>[2x]GMAGGRGAPGRGRDEPPESYPQRQDHELQALEAIYGADFQDLRPDACGPVKEPPEINLVLYPQGLTGEEVYV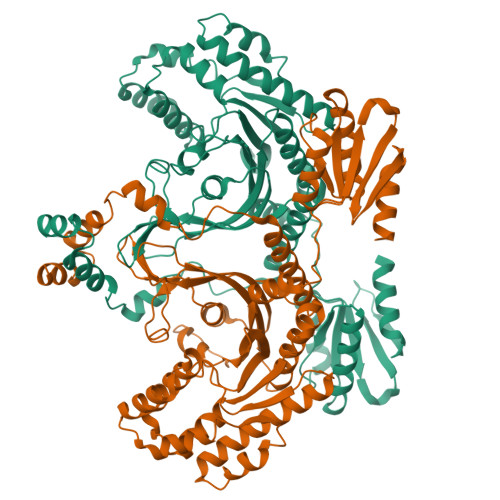KVDLRVKCPPTYPDVVPEIELKNAKGLSNESVNLLKSRLEELAKKHCGEVMIFELAYHVQSFLSEHNKPPPKSFHEEMLERRAQEEQQRLLEAKRKEEQEQREILHEIQRRKEEIKEEKKRKEMAKQERLEIASLSNQDHTSKKDPGGHRTAAILHGGSPDFVGNGKHRANSSGRSRRERQYSVCNSEDSPGSCEILYFNMGSPDQLMVHKGKCIGSDEQLGKLVYNALETATGGFVLLYEWVLQWQKKMGPFLTSQEKEKIDKCKKQIQGTETEFNSLVKLSHPNVVRYLAMNLKEQDDSIVVDILVEHISGVSLAAHLSHSGPIPVHQLRRYTAQLLSGLDYLHSNSVVHKVLSASNVLVDAEGTVKITDYSISKRLADICKEDVFEQTRVRFSDNALPYKTGKKGDVWRLGLLLLSLSQGQECGEYPVTIPSDLPADFQDFLKKCVCLDDKERWSPQQLLKHSFINPQPKMPLVEQSPEDSEGQDYVETVIPSNRLPSAAFFSETQRQFSRYFIEFEELQLLGKGAFGAVIKVQNKLDGCCYAVKRIPINPASRQFRRIKGEVTLLSRLHHENIVRYYNAWIERHERPAGPGTPPPDSGPLAKDDRAARGQPASDTDGLDSVEAAAPPPILSSSVEWSTSGERSASARFPATGPGSSDDEDDDEDEHGGVFSQSFLPASDSESDIIFDNEDENSKSQNQDEDCNEKNGCHESEPSVTTEAVHYLYIQMEYCEKSTLRDTIDQGLYRDTVRLWRLFREILDGLAYIHEKGMIHRDLKPVNIFLDSDDHVKIGDFGLATDHLAFSADSKQDDQTGDLIKSDPSGHLTGMVGTALYVSPEVQGSTKSAYNQKVDLFSLGIIFFEMSYHPMVTASERIFVLNQLRDPTSPKFPEDFDDGEHAKQKSVISWLLNHDPAKRPTATELLKSELLPPPQMEESELHEVLHHTLTNVDGKAYRTMMAQIFSQRISPAIDYTYDSDILKGNFSIRTAKMQQHVCETIIRIFKRHGAVQLCTPLLLPRNRQIYEHNEAALFMDHSGMLVMLPFDLRIPFARYVARNNILNLKRYCIERVFRPRKLDRFHPKELLECAFDIVTSTTNSFLPTAEIIYTIYEIIQEFPALQERNYSIYLNHTMLLKAILLHCGIPEDKLSQVYIILYDAVTEKLTRREVEAKFCNLSLSSNSLCRLYKFIEQKGDLQDLMPTINSLIKQKTGIAQLVKYGLKDLEEVVGLLKKLGIKLQVLINLGLVYKVQQHNGIIFQFVAFIKRRQRAVPEILAAGGRYDLLIPQFRGPQALGPVPTAIGVSIAIDKISAAVLNMEESVTISSCDLLVVSVGQMSMSRAINLTQKLWTAGITAEIMYDWSQSQEELQEYCRHHEITYVALVSDKEGSHVKVKSFEKERQTEKRVLETELVDHVLQKLRTKVTDERNGREASDNLAVQNLKGSFSNASGLFEIHGATVVPIVSVLAPEKLSASTRRRYETQVQTRLQTSLANLHQKSSEIEILAVDLPKETILQFLSLEWDADEQAFNTTVKQLLSRLPKQRYLKLVCDEIYNIKVEKKVSVLFLYSYRDDYYRILF> MKLLTHNLLSSHVRGVGSRGFPLRLQATEVRICPVEFNPNFVARMIPKVEWSAFLEAADNLRLIQVPKGPVEGYEENEEFLRTMHHLLLEVEVIEGTLQCPESGRMFPISRGIPNML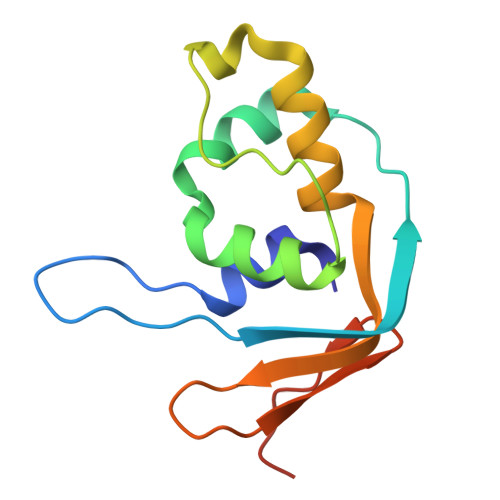LSEEETES> AAAAAAAAAAAAAAAAAAAAAAA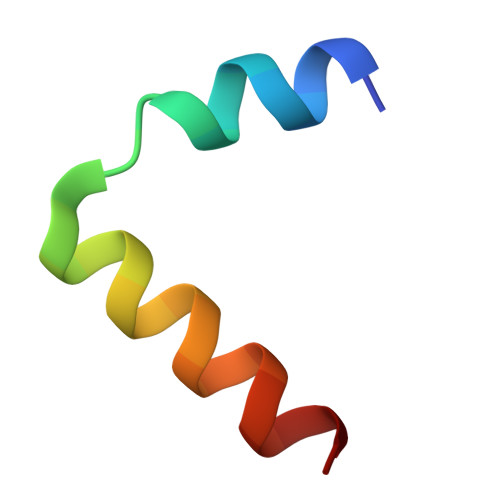AAAAA>[12x]MVLILNGPNLNLLGRREPEVYGRTTLEELEALCEAWGAELGLGVVFRQTNYEGQLIE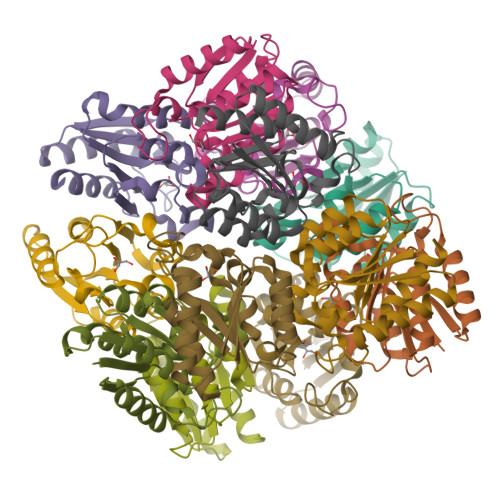WVQQAHQEGFLAIVLNPGALTHYSYALLDAIRAQPLPVVEVHLTNLHAREEFRRHSVTAPACRGIVSGFGPLSYKLALVYLAETLEVGGEGF4-HYDROXYBENZALDEHYDE 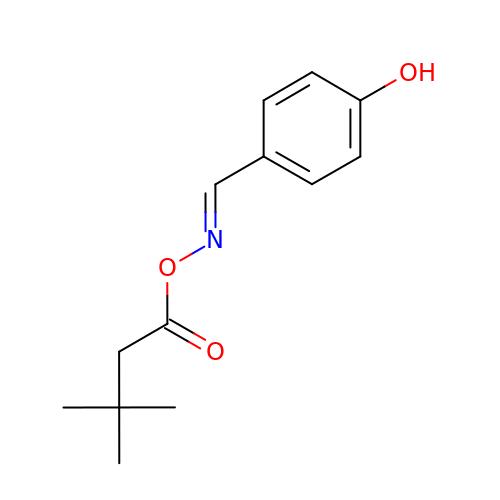O-(3,3-DIMETHYLBUTANOYL)OXIME | C13 H17 N O3 | IRHAIEVALGHVLW-NTEUORMPSA-N> GSTIYHAKDAVQATKPDMRKPRLVVFVVGETARADHVSFNGYERDTFPQLAKIDGVTNFSNVTSCGTSTAYSVPCMFSYLGADEYDVDTAKYQENVLDTLDRLGVSILWRDNNSDSKGVMDKLPKAQFADYKSATNNAICNTNPYNECRDVGMLVGLDDFVAANNGKDMLIMLHQMGNHGPAYFKRYDEKFAKFTPVCEGNELAKCEHQSLINAYDNALLATDDFIAQSIQWLQTHSNAYDVSMLYVSDHGESLGENGVYLHGMPNAFAPKEQRSVPAFFWTDKQTGITPMATDTVLTHDAITPTLLKLFDVTADKVKDRTAFIR

Based on sequence alignment, MCR-1 should be a phosphoethanolamine transferase, a member of YhjW/YjdB/YijP superfamily which catalyzes the addition of phosphoethanolamine to lipid A moiety of lipopolysaccharides (LPS) and therefore confers colistin resitance to its host. MCR-1 contains two domains, one N-terminal transmembrane domain and one periplasmic C-terminal catalytic domain33. The newly identified mcr-1 is a mobile colistin resistant gene and has been shown to rapidly spread among various bacterial strains through horizontal transfer and assisted its host in colistin resistance.

To understand the molecular mechanism of colistin resistance and structural features, here we report the X-ray structure of the C-terminal catalytical domain of MCR-1 (aa: 219–541, MCR-1C for short) determined at 1.45 Å resolution. The protein was crystallized in space group P212121 having one MCR-1C molecule in the asymmetric unit with a solvent content of 42.5%. The structure was solved by single-wavelength anomalous scattering (SAD) method using the anomalous signal of zinc ions with well-defined electron density map for all the residues in the construct. The MCR-1C adopted an α/β/α topology with seven β-strands, sandwiched between two layers of α-helices. MCR-1C consists of three disulfide bridges as revealed in the crystal structure (shown as ball-and-stick models). The Cys414-Cys422 bridge stabilized a loop (aa: Lys409-Glu423) located at the top of the protein whereas Cys281-Cys291 completes the catalytic site by locking a smaller α-helix (aa: Thr285-Met292) to the central β sheet. The third disulfide bridge Cys356-Cys364 is only shared between MCR-1C and LptA and it seems to arrest the conformational freedom of the loop (aa: Lys348–365) and facilitate substrate entry. In our study among the three identified zinc ions in MCR-1C, two of them were located at the active site and the third one located near residue Cys291. Similar to LptA and EptC, the first zinc ion (Zn1) is highly conserved in active site contacts and is coordinated to residues Glu246, Thr285, Asp465 and His466333444. The phosphorylated Thr285 is considered a catalysis intermediate during phosphate transfer thus stating MCR-1C the first native structure without any bound substrate or reaction intermediate.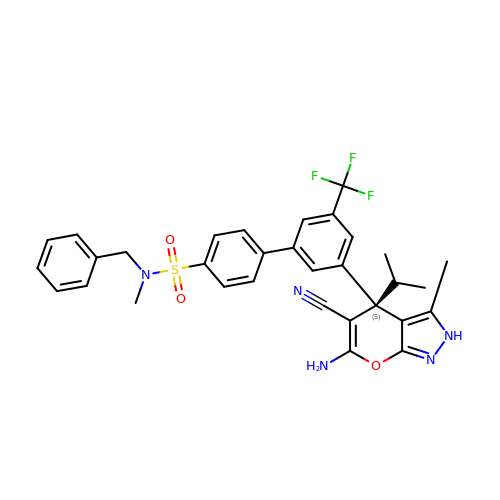4-[3-[(4~{S})-6-azanyl-5-cyano-3-methyl-4-propan-2-yl-2~{H}-pyrano[2,3-c]pyrazol-4-yl]-5-(trifluoromethyl)phenyl]-~{N}-methyl-~{N}-(phenylmethyl)benzenesulfonamide | C32 H30 F3 N5 O3 S | DBROLDANENNIQJ-HKBQPEDESA-N> DLYFQSHMTIAVTGSIATDHLMRFPGRFSEQLLPEHLHKVSLSFLVDDLVMHRGGVAGNMAFAIGVLGGEVALVGAAGADFADYRDWLKA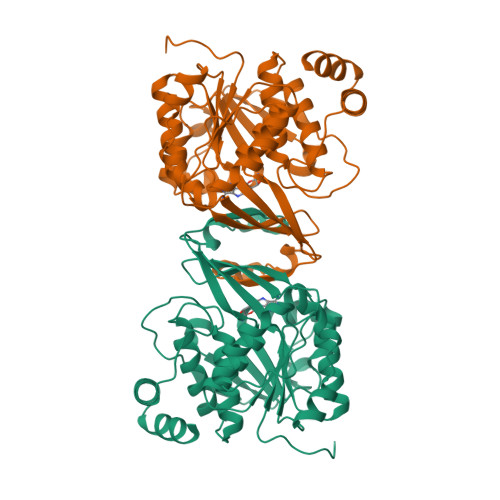RGVNCDHVLISETAHTARFTCTTDVDMAQIASFYPGAMSEARNIKLADVVSAIGKPELVIIGANDPEAMFLHTEECRKLGLAFAADPSQQLARLSGEEIRRLVNGAAYLFTNDYEWDLLLSKTGWSEADVMAQIDLRVTTLGPKGVDLVEPDGTTIHVGVVPETSQTDPTGVGDAFRAGFLTGRSAGLGLERSAQLGSLVAVLVLESTGTQEWQWDYEAAASRLAGAYGEHAAAEIVAVLA> MCDLPQTHSLGSRRTLMLLAQMRRISLFSCLKDRHDFGFPQEEFGNQFQKAETIPVLYNMISQIFNLFSTKDSSAAWDETLLDKFYTELYQQLNDLEACVIQGVGVTETPLMKEDSILAVRKYFQRITLYLKEKKYSPCAWEVVRAEIMRSFSLSTNLQESLRSK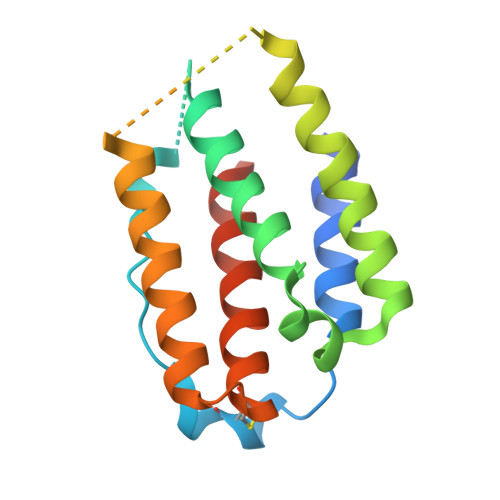E> SPKR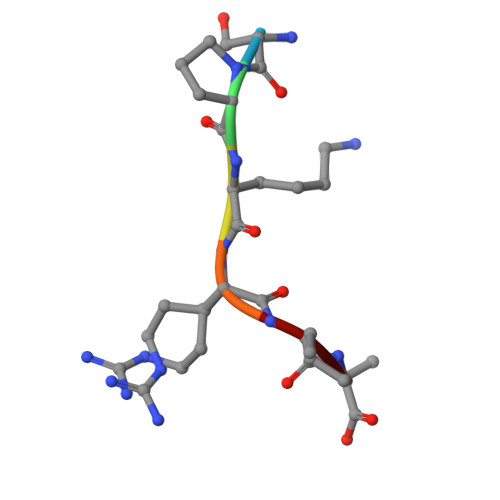IA>MKHSLPDLPYDYGALEPHINAQIMQLHHSKHHAAYVNNLNVTEEKYQEALAKGDVTAQIALQPALKFNGGGHINHSIFWTNLSPNGGGEPKGELLEAIKRDFGSFDKFKEKLTAASVGVQGSGWGWLGFNKERGHLQIAACPNNDPLQGTTGLIPLLGIDVWEHAYYLQYKNVRPDYLKAIWNVINWENVTERYMACKK[2x]

Human manganese superoxide dismutase (MnSOD) is a mitochondrial matrix metalloenzyme that catalyzes the dismutation of reactive superoxide radicals, generated as byproducts of mitochondrial respiration, into molecular oxygen (O2) and hydrogen peroxide (H2O2). As the only known mitochondrial enzyme capable of converting reactive radicals into diffusible products that can be further metabolized or exported, MnSOD serves as the critical first line of defence against oxidative stress. In the wild-type enzyme, Gln143 mediates proton transfers with the manganese-bound solvent (WAT1) to drive redox cycling of the metal, which is necessary for effective superoxide dismutation. Substitution with Asn stalls catalysis because the increased distance from WAT1 disrupts critical proton-coupled electron-transfer (PCET) events, and the redox cycling of the active-site metal is impaired.

Substituting Gln143 with Asn preserves the active-site architecture, but the hole created disrupts proton transfers with the WAT1 solvent. The alternate Tyr34 conformation and the presence of the Wcav solvent introduce new hydrogen bonds within the active site of Gln143Asn MnSOD, which are not observed in the wild-type enzyme. We note that the resting-state electrostatic solvent-accessible surface of Gln143Asn MnSOD is different from the surface of resting-state wild-type MnSOD. The active-site funnel of the wild type is much more positively charged than that of the Gln143Asn mutant. This is because the wild-type resting state contains Mn3+ and the Gln143Asn resting state contains Mn2+. Gln143Asn MnSOD retains the more neutral surface most of the time, and this seems to help stabilize the H2O2-binding sites. To monitor changes in the oxidation state and coordination geometry of the catalytic manganese in the Gln143Asn variant upon H2O2 treatment, we compared the Mn K-edge high-energy-resonance fluorescence-detected X-ray absorption near-edge spectra (HERFD-XANES) of the purified enzyme before and after H2O2 treatment, following established protocols. We observe no detectable shift in either rising-edge or pre-edge features, indicating no alteration in the redox state or coordination geometry of the catalytic manganese after H2O2 treatment in Gln143Asn MnSOD.> MSTSTEKRSKENLPWVEKYRPETLDEVYGQNEVITTVRKFVDEGKLPHLLFYGPPGTGKTSTIVALAREIYGKNYSNMVLELNASDDRGIDVVRNQIKDFASTRQIFSKGFKLIILDEADAMTNAAQNALRRVIERYTKNTRFCVLAN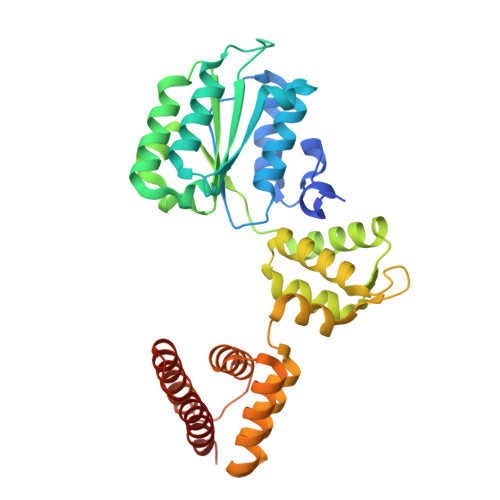YAHKLTPALLSRCTRFRFQPLPQEAIERRIANVLVHEKLKLSPNAEKALIELSNGDMRRVLNVLQSCKATLDNPDEDEISDDVIYECCGAPRPSDLKAVLKSILEDDWGTAHYTLNKVRSAKGLALIDLIEGIVKILEDYELQNEETRVHLLTKLADIEYSISKGGNDQIQGSAVIGAIKASFENETVKAN> MAPSFDHLREEDLDEEDIDMDEVDISDLREKYEVQLEQGYDTFVVIDGLPAVSEEQKPKLIKFLLKKLNTVGKTREDMIYMPMGDDGMSLRFAFVEYSSPAEASAAVRQLDYVPLDKKHTLRVNKLTDIDRYGREGRISEEFVPPKIEPFQEKEHLRWFMADPADRGRDQFVMYRGDTVGVFWNNEKDQPENIVDRQHWTETFVQWSPLGTYLTSVHAQGVQLWGGASWSRLRRFPHPFVNLVAFSPGEKYLVTWSNRPIQIPDSGHPVLTLDDDGKNYIIWDIETARPLRSFAQQDIHPEEHGPKKGPPKFPWPVFKWSADDKYVARLNQGTSISIYELPKMNLLDKQAVKIEGVMDFEWAPATVQREGVKTYEQLFCFWTPEIGNNPARVGLMSIPS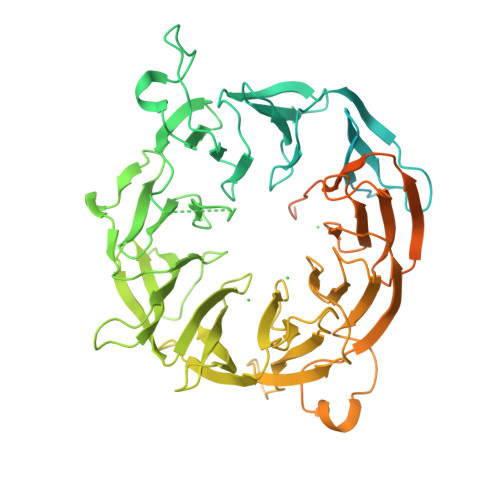KQIVRTLNLFSVSDVKMHWQSEGTYLCVKVDRHSKSKKSQATTLEIFRVKEKGVPVEVVDTIKDTVINFAWEPKGDRFVIITTPEPVGATAVPPKTSVSFFCPELKKGNQVGSFKHLRTLEKKNHNAIYWSPKGRFVVIATVHNTQSSDLEFWDLDFDGEKPENEKDLAACLQLMGTGDHYGITDVEWDPSGRYVATWASAWKHTMENGYHLYDFKGELLREEHIEKFKQWQWRPRPPTLLTKEEQKQIRKNLREYSRIFEQEDAERISSADVAVVEARRRLLNEWYAWREAIEKEVAEERAALGLPADPAAELLKRKIAEVAPDAQEQVIEEIMEEVLEETEEIVN> MSEIGTGFPFDPHYVEVLGERMHYVDVGP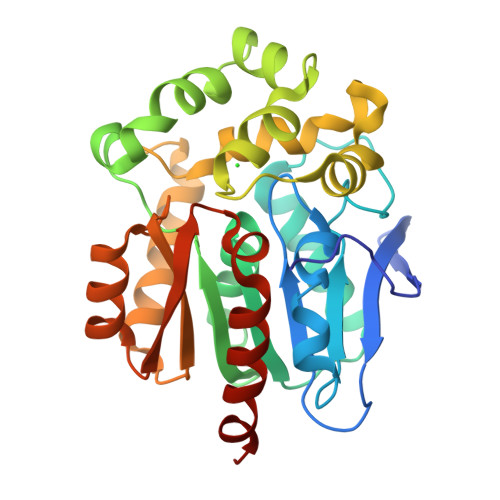RDGTPVLFLHGNPTSSYLWRNIIPHVAPSHRCIAPDLIGMGKSDKPDLDYFFDDHVRYLDAFIEALGLEEVVLVIHDWGSALGFHWAKRNPERVKGIACMEFIRPIPTWDEWPEFARETFQAFRTADVGRELIIDQNAFIEGALPKCVVRPLTEVEMDHYREPFLKPVDREPLWRFPNELPIAGEPANIVALVEAYMNWLHQSPVPKLLFWGTPGVLIPPAEAARLAESLPNCKTVDIGPGLHYLQEDNPDLIGSEIARWLPALHHHHHH> MGSVQRQDLVLFSDQSVLPAHFFQDSNSHNLFFITHQSCTQPLWMINALVETHVLGSPSSLNESSSSMLPSSTRSHAVLASFIHEQNYFTNSLNKLKIPSNNYNVLDFLSDFIVNNIHNKPRDKILSDVLAKFSAAIQNNPTDTIVIIEQPELLLSLVSGLTCSELNNKFITPLLRQCKVLIIVSNSDIFNIDEYDASVHSSNLQNFYKSSFIKS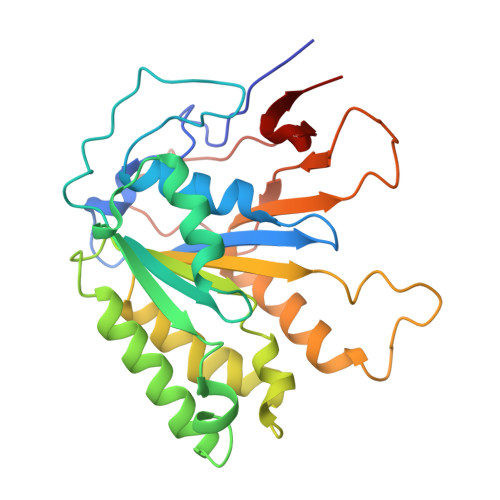MINLNLNPLKTGFAKDVTGSLHVCRGGAPIATSNTSLHVVENEYLYLNEKESTKLFYR>MRSMKALQKALSRAGSHCGRGGWGHPSRSPLLGGGVRHHLSEAAAQGRETPHSHQPQHQDHDSSESGMLSRLGDLLFYTIAEGQERIPIHKFTTALKATGLQTSDPRLRDCMSEMHRVVQESSSGGLLDRDLFRKCVSSNIVLLTQAFRKKFVIPDFEEFTGHVDRIFEDVKELTGGKVAAYIPQLAKSNPDLWGVSLCTVDGQRHSVGHTKIPFCLQSCVKPLTYAISISTLGTDYVHKFVGKEPSGLRYNALSLNEEGIPHNPMVNAGAIVVSSLIKMDCNKAEKFDFVLQYLNKMAGNEYMGFSNATFQSEKETGDRNYAIGYYLKEKKCFPKGVDMMAALDLYFQLCSVEVTCESGSVMAATLANGGICPITGESVLSAEAVRNTLSLMHSCGMYDFSGQFAFHVGLPAKSAVSGAILLVVPNVMGMMCLSPPLDKLGNSHRGTSFCQKLVSLFNFHNYDNLRHCARKLDPRREGAEIRNKTVVNLLFAAYSGDVSALRRFALSAMDMEQKDYDSRTALHVAAAEGHIEVVKFLIEACKVNPFAKDRWGNIPLDDAVQFNHLEVVKLLQDYQDSYTLSETQAEAAAEALSKENLESMV[12x]

The glutaminase enzymes GAC and GLS2 catalyze the hydrolysis of glutamine to glutamate, satisfying the ‘glutamine addiction’ of cancer cells. All glutaminase enzymes share a catalytic domain containing identical active site residues and a conserved mechanism for hydrolyzing glutamine to glutamate. Here we demonstrate that the ability of GAC and GLS2 to form filaments is directly coupled to their catalytic activity and present their cryo-EM structures which provide a view of the conformational states essential for catalysis. Filament formation guides an ‘activation loop’ to assume a specific conformation that works together with a ‘lid’ to close over the active site and position glutamine for nucleophilic attack by an essential serine.

We also obtained a 3.3 Å cryo-EM structure of the constitutively active recombinant human GLS2 (K253A) mutant that formed a filament immediately after the addition of glutamine alone (and prior to substrate depletion), as this mutant does not require an anionic activator to be catalytically competent. The tetramers are arranged in a side-by-side architecture and each successive tetramer is rotated ~48 degrees relative to the filament axis, with the helical rise of ~66 Å. Interestingly, in the filament structure for the constitutively active GLS2 mutant, Arg320 (which corresponds to Arg387 in GAC) forms the same type of salt bridge in the absence of Pi, as that seen when Pi binds to GAC(Y466W). The formation of these Arg-Glu salt bridges, together with the substitution of a less bulky alanine residue for lysine, allows the movement of the activation loops into a space that otherwise would only occur when Pi binds, and likely explains why the Lys-to-Ala substitutions within the loops yield enzymes that no longer require the binding of an anionic activator. An additional conformational change that occurs specifically in the constitutively active GLS2 filament structure, when compared to the tetrameric apo-enzyme, results in a hydrogen bonding network introduced by the activation loops. Hydrogen bonds that form between Arg250 and Asp400 of GLS2 appear to ‘stretch’ the alpha helix containing Asp400, causing Tyr399 on the N-terminal end of the alpha helix to insert further into the active site where the substrate binds. Following the insertion of Tyr399, Glu258 from the adjacent dimer forms a hydrogen bond with Lys440, which displaces the loop containing Lys440, and therefore makes space for the insertion of Tyr399. As a result, Tyr399 is now in close proximity to both Lys222 and the substrate, which is necessary for catalysis.>[2x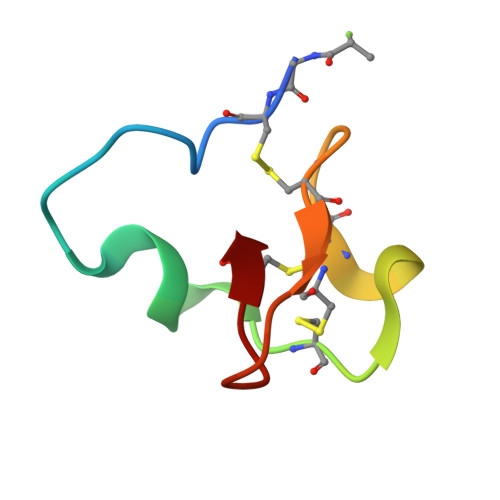]XGCILNGRTDLGTLLFRCRRDSDCPGACICRGNGYCG>MVHSSAMVNSHRKPMFNIHRGFYCLTAILPQICICSQFSVPSSYHFTEDPGAFPVATNGERFPWQELRLPSVVIPLHYDLFVHPNLTSLDFVASEKIEVLVSNATQFIILHSKDLEITNATLQSEEDSRYMKPGKELKVLSYPAHEQIALLVPEKLTPHLKYYVAMDFQAKLGDGFEGFYKSTYRTLGGETRILAVTDFEPTQARMAFPCFDEPLFKANFSIKIRRESRHIALSNMPKVKTIELEGGLLEDHFETTVKMSTYLVAYIVCDFHSLSGFTSSGVKVSIYASPDKRNQTHYALQASLKLLDFYEKYFDIYYPLSKLDLIAIPDFAPGAMENWGLITYRETSLLFDPKTSSASDKLWVTRVIAHELAHQWFGNLVTMEWWNDIWLNEGFAKYMELIAVNATYPELQFDDYFLNVCFEVITKDSLNSSRPISKPAETPTQIQEMFDEVSYNKGACILNMLKDFLGEEKFQKGIIQYLKKFSYRNAKNDDLWSSLSNSCLESDFTSGGVCHSDPKMTSNMLAFLGENAEVKEMMTTWTLQKGIPLLVVK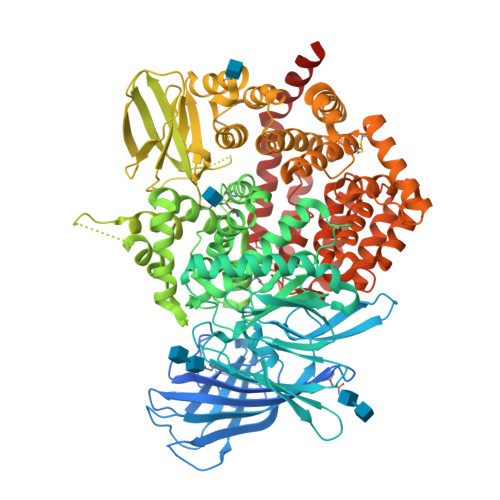QDGCSLRLQQERFLQGVFQEDPEWRALQERYLWHIPLTYSTSSSNVIHRHILKSKTDTLDLPEKTSWVKFNVDSNGYYIVHYEGHGWDQLITQLNQNHTLLRPKDRVGLIHDVFQLVGAGRLTLDKALDMTYYLQHETSSPALLEGLSYLESFYHMMDRRNISDISENLKRYLLQYFKPVIDRQSWSDKGSVWDRMLRSALLKLACDLNHAPCIQKAAELFSQWMESSGKLNIPTDVLKIVYSVGAQTTAGWNYLLEQYELSMSSAEQNKILYALSTSKHQEKLLKLIELGMEGKVIKTQNLAALLHAIARRPKGQQLAWDFVRENWTHLLKKFDLGSYDIRMIISGTTAHFSSKDKLQEVKLFFESLEAQGSHLDIFQTVLETITKNIKWLEKNLPTLRTWLMVNTRHHHHHH[2x]> MTDKHYARVVDGLVVETKTLPADFNLDDLFGP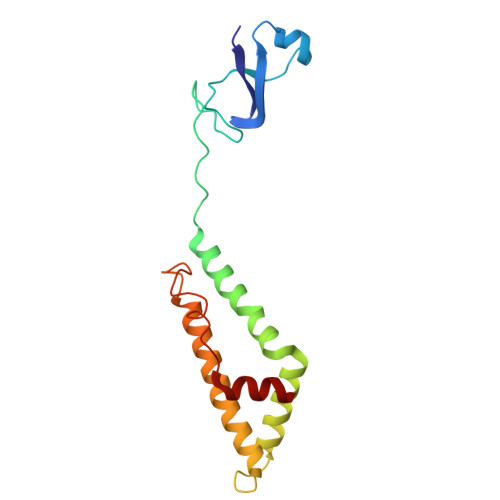DHGWVEAPLEVEQGWRKVGAKFAPAPPPERDPASILAGLKAEASRHIFATISATAQSNLLLAVGLASAKAPSARTPEERDLLNVADEGRAWIDAVRARVHALAEHDGVTPKGEDRWPAPSEAVLEMAAKF> EKLGKLQYSLDYDFQNNQLLVGIIQAAELPALDMGGTSDPYVKIHLMQNGKRLKKKKTTIKKNTLNPVFNEQFTFKVPYSELGGKTLVMAVYDFDRFSKHDI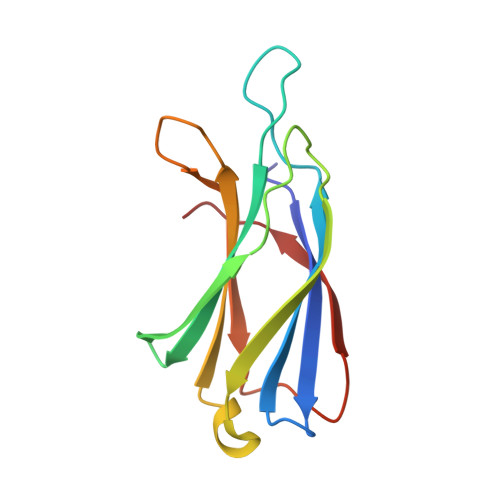IGEFKVPMNTVDFGHVTEEWRDLQSA>NANRSKEWKNAANTLLFGLDESVDPCEDFYGFTCNKFIERIDLDELGRGRFTTFSQAQLEVNSDIVKALEKVDVNDEKFSQTERITKAAFQSCVEYTLKDDRKASVNELLQYISERFGGIPFLGQRVKGGCELYREMGRIEQQRALPTFMYTWVNVDHKNVSRNSYYISQ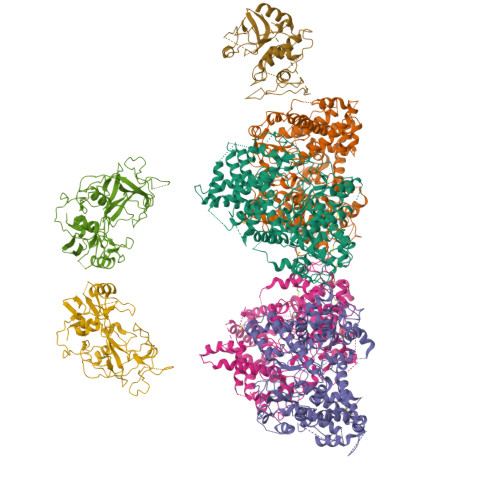PTLPMPREFYVLPQFAPELDARTKAIENVMKAFASDILKDPSKYDKMIKTAAREVTQIEQKIAMASWPDDELRNHEQQYNPYELFAPSEGKIALQDAFPNIRFGKYIAGLMETATGGVPVSPVFIGDVIVTNPAYMGFLNTLFRQTNIQMNQYPFVNYIIVHMLFEDAEHLGDKYLRIAKDADYVTYAQRKGVGITRSGRKYSRVFDERTDARMKCVDTITTYMPYGTGYVYVNSREDRDQVVEDVKQQTELIMKTFLKKMLSTLSWMQGESYRRAEKKINEMHRNYGWPKKLFGDFKNFDTIDAYHRDDYYSILEAYNNKTDKSTAFYTILNILRRGYENRESFRRKNETADRTNFLESPASVNAWYAPELNSLTLPFGILTSPHYDLQFPKAFNFAGSGTVGGHELVHGFDDEGVQFDYDGSLADCSVYECGWLEQKGKNGFKDMAQCVVTQYNAQCCPAKEGNVHCANGAHTQGENIADLGGLQASYNAYKEYIKMKGAEEMRLPGLEKFTPNQIFWISYGYSWCAKETQSSLVKRLLTNPHSPNSCRVNQVLQDIPSFAKDFQCALGQKMYPPAEQRCKVW[4x];>VFPHPIYDYQDTEYLAKITIGAPGQSFHVVLDTGSANLWIPDNICVNGRRGACRITTCDRGLVCEVLCHDKSCCEDDVDNPDEDNPCKGKSGFDSTQSTSYAKITPKKYFEIVYGTGFAKGFLGNDTVRFGEEGNNKTLVVPGTVFGQAVQIGDPFANNPINGILGLGFRGLAQAGVTPPLQRAIDLKLVDPIFTVYMKQLGAKAKGQDGGAFTYGGLDSVNCGQEIAYVDLTRPLYWQFKMEAFSAGYLSIRKGWEVISDTGTSFMGVPTAIADLVADSYGGQYDEMFEIYTVDCNATVTFGMTIGGKQYKIERKNLVLEEDKDSCMIAMTPLSSVGFGPQWILGAPFIRQYCNIHDMRNNTIGFAEP[2x];> DPDIPENYDPRLIWPNCSSLFTIPDQANCGSCWAVSTAAAISDRLCIASKGENQVFISSADILSCCDTCGFGCDGGITFRAWEYFATKGSVSGGHFEAPNCCRPYYFHPCGQHGNDTFYGYCPRFAQTPFCRRKCRIGFNKSYAQDRIQGKSFYTVDYSVPAIQREIMTKGSVVGSYDVFTDFSHYKSGIYRHTGGKPDGRHAVRIIGWGKENGTDYWLIANSWHDDWGENGYFRMIRGINDCGIEQDITAGD We report the development of three ubiquitin variants (UbVs), each binding selectively to the RING or U-box domain of a distinct E3 ligase: monomeric UBE4B, phosphorylated active CBL, or dimeric XIAP. With ∼600 members, the RING/U-box E3s form the largest family. This family uses a RING or U-box domain to recruit E2 enzymes thioesterified with Ub (E2∼Ub) and facilitates transfer of Ub directly to substrate. RING/U-box domains promote Ub transfer by shifting the equilibrium of E2∼Ub into a closed conformation (Dou et al., 2012b, Plechanovová et al., 2012, Pruneda et al., 2012). We generated selective UbVs for each RING/U-box domain and used biochemical assays and structural studies to identify two types of UbVs: competitive inhibitors of E2∼Ub binding sites on UBE4B or phosphorylated CBL and an activator of XIAP.

UBE4B is known as a Ub elongation factor or E4 because it binds preformed Ub conjugates and catalyzes formation of polyubiquitin chains (Kaneko et al., 2003, Koegl et al., 1999). UbV.E4B selectively inhibited E4B, the U-box domain of UBE4B. We attempted to co-crystallize UbV.E4B with several E4B U-box variants of differing lengths. A crystal structure of UBE4B U-box comprising residue 1,097 to the C terminus (E4B1097–C) was determined to a resolution of 1.48 Å, but no crystals of a complex with UbV.E4B were obtained. We therefore undertook nuclear magnetic resonance (NMR) experiments to map the complex interface. To investigate whether UbV.E4B and E2 compete for the same binding site on E4B, we monitored CSPs in 15N-UbcH5B competition experiments. Addition of equimolar E4B to 15N-UbcH5B strongly affected several residue peaks within the spectra indicating formation of 15N-UbcH5B-E4B complex. Subsequent titration of UbV.E4B caused 15N-UbcH5B signals to shift back to free E2 positions, showing that UbV.E4B inhibits E4B by occupying the E2-binding site.

> GSDAPDEFRDPLMDTLMTDPVRLPSGTIMDRSIILRHLLNSPTDPFNRQTLTESMLEPVPELKEQIQAWMREKQNSDH> MEILEEKPKEGKVKVKAETLDDLWHLYHIIDPGDIVYAKTLRKQAQRADSLRAEKVEVIPVFLGVQAEKINFHKFANQVRVTGPIVYASREDVPLGKYHTIAIEQGTVVTIQKPRWKEHHIERLKEAVAASKRARVMIVVIDDGEADMALVREYGVEILNSIRHNLGGKRYNTDRESEEMKFFHDVAKTMEEVMKRENVEKAIVAGPGFVKEDFYKFLKEKYPELAKKVVIEDTSVTGRTGIYEVIKRGVVDRVYQENRVAKEVQLVEKVLENIARNNGLVAYGLKEVEEAVNYGAVETLLVLDELLKGELREKVEELMDAVRYSRGEVVVVSSEHEGGEKLKALGGLAALLRFRVK;> MVRKMRIAVIDYDKCNPDKCGHFLCERVCPVNRMGGEAIIIDEENYKPIIQEASCTGCGICVHKCPFNAISIVNLPEQLDEDCVHRYGVNAFVLYRLPIVKDGMVVGIVGPNGTGKTTAVKILAGQLIPNLCEDNDSWDNVIRAFRGNELQNYFERLKNGEIRPVVKPQYVDLLPKAVKGKVRELLKKVDEVGKFEEVVKELELENVLDRELHQLSGGELQRVAIAAALLRKAHFYFFDEPSSYLDIRQRLKVARVIRRLANEGKAVLVVEHDLAVLDYLSDVIHVVYGEPGVYGIFSKPKGTRNGINEFLQGYLKDENVRFRPYEIRFTKLSERVDVERETLVEYPRLVKDYGSFKLEVEPGEIRKGEVIGIVGPNGIGKTTFVKMLAGVEEPTEGKVEWDLTVAYKPQYIKAEYEGTVYELLSKIDSSKLNSNFYKTELLKPLGIIDLYDRNVEDLSGGELQRVAIAATLLRDADIYLLDEPSAYLDVEQRLAVSRAIRHLMEKNEKTALVVEHDVLMIDYVSDRLIVFEGEPGRHGRALPPMGMREGMNRFLASVGITFRRDPDSGRPRANKEGSVKDRE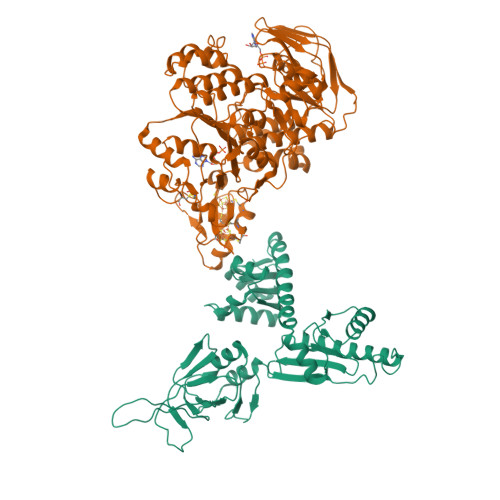QKARGEYYYA>MRGSHHHHHHTDPSNYGKSADGTVTIEYFNQKKEMTKTLEEITRDFEKENPKIKVKVVNVPNAGEVLKTRVLAGDVPDVVNIYPQSIELQEWAKAGVFEDLSNKDYLKRVKNGYAEKYAVNEKVYNVPFTANAYGIYYNKDKFEELGLKVPETWDEFEQLVKDIVAKGQTPFGIAGADAWTLNGYNQLAFATATGGG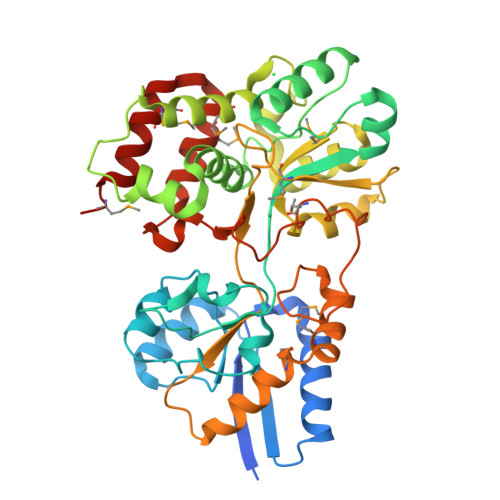KEANQYLRYSQPNAIKLSDPIMKDDIKVMDILRINGSKQKNWEGAGYTDVIGAFARGDVLMTPNGSWAITAINEQKPNFKIGTFMIPGKEKGQSLTVGAGDLAWSISATTKHPKEANAFVEYMTRPEVMQKYYDVDGSPTAIEGVKQAGEDSPLAGMTEYAFTDRHLVWLQQYWTSEADFHTLTMNYVLTGDKQGMVNDLNAFFNPMKADVD[2x]6-sulfanylidene-1,7-dihydropyrazolo[3,4-d]pyrimidin-4-one 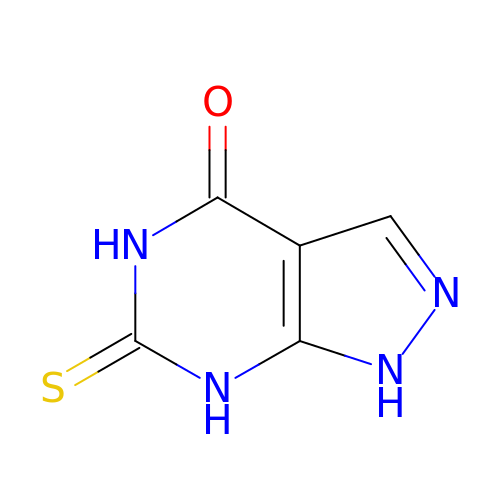| C5 H4 N4 O S | SXRSXYWROQWSGJ-UHFFFAOYSA-N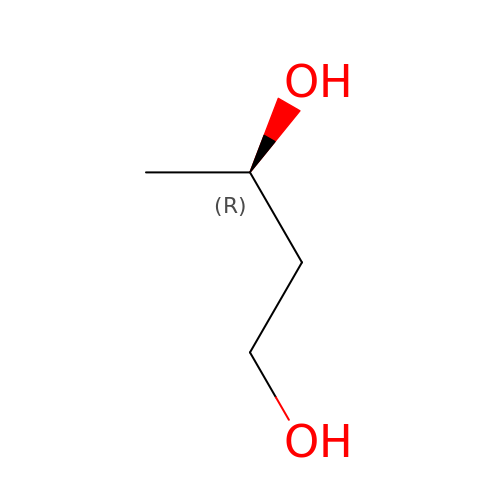(3R)-butane-1,3-diol | C4 H10 O2 | PUPZLCDOIYMWBV-SCSAIBSYSA-N N-(4-methoxyphenyl)-N~2~-[1-(2-methylphenyl)-4-oxo-4,5-dihydro-1H-pyrazolo[3,4-d]pyrimidin-6-yl]-L-alaninamide 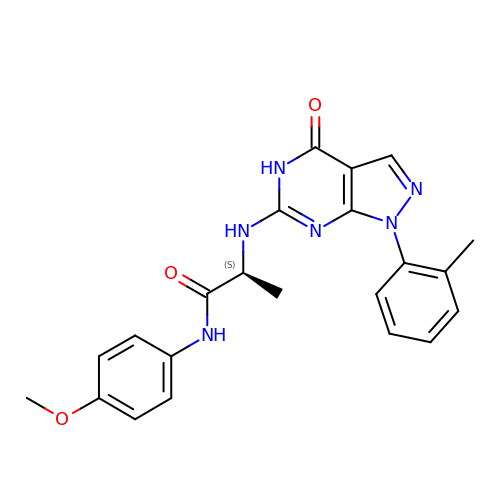| C22 H22 N6 O3 | VHGPQZWYIWLLDA-AWEZNQCLSA-N>MKSPEEIKGAFEVFAAKEGDPNQISKEELKLVMQTLGPSLLKGMSTLDEMIEEVDKNGDGEVSFE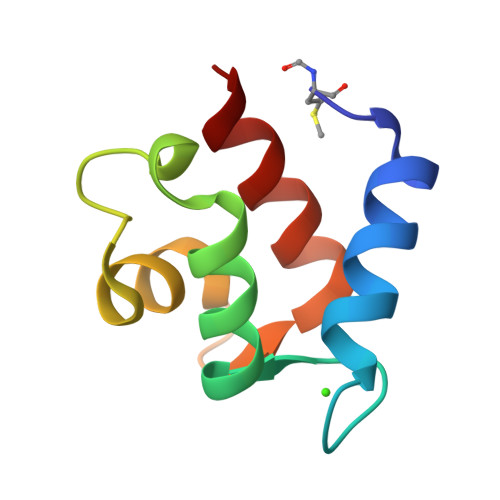EFLVMMKKISQ[2x]>[2x]ANDIDNSNPVVQAEQLNWLHYLMNYGSIVANDPEANFDGVRVDAVDNVNADLLQIASDYLKAHYGVDKSEKNAINHLSILEAWSDNDPQYNKDTKGAQLPIDNKLRLSLLYALTRPLEKDASNKNEIRSGLEPVITNSLNNRSAEGKNSERMANYIFIRAHDSEVQTVIAKIIKAQINPKTDGLTFTLDELKQAFKIYNEDMRQAKKKYTQSNIPTAYALMLSNKDSITRLYYGDMYSDDGQYMATKSPYYDAIDTLLKARIKYAAGGQDMKITYVEGDKSHMDWDYTGVLTSVRYGTGANEATDQGSEATKTQGMAVITSNNPSLKLNQNDKVIVNMGTAHKNQEYRPLLLTTKDGLTSYTSDAAAKSLYRKTNDKGELVFDASDIQGYLNPQVSGYLAVWVPVGASDNQDVRVAASNKANATGQVYESSSALDSQLIYEGFSNFQDFVTKDSDYTNKKIAQNVQLFKSWGVTSFE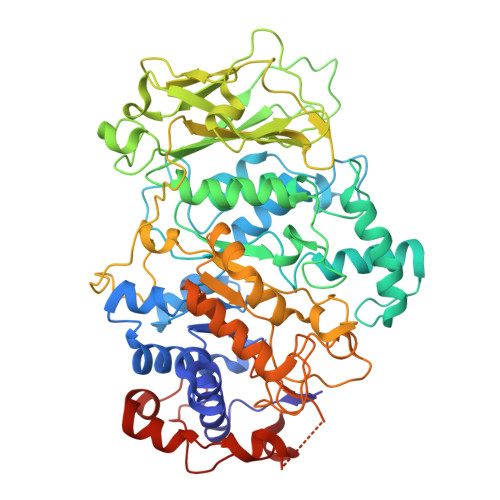MAPQYVSSEDGSFLDSIIQNGYAFEDRYDLAMSKNNKYGSQQDMINAVKALHKSGIQVIADWVPDQIYNLPGKEVVTATRVNDYGEYRKDSEIKNTLYAANTKSNGKDYQAKYGGAFLSELAAKYPSIFNRTQISNGKKIDPSEKITAWKAKYFN>AESCTSRPHITVVEGEPFYLKHCSCSLAHEIETTTKSWYKSSGSQEHVELNPRSSSRIALHDCVLEFWPVELNDTG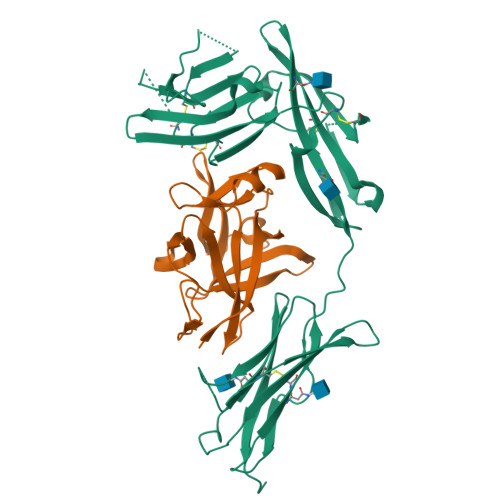SYFFQMKNYTQKWKLNVIRRNKHSCFTERQVTSKIVEVKKFFQITCENSYYQTLVNSTSLYKNCKKLLLENNKNPTIKKNAEFEDQGYYSCVHFLHHNGKLFNITKTFNITIVEDRSNIVPVLLGPKLNHVAVELGKNVRLNCSALLNEEDVIYWMFGEENGSDPNIHEEKEMRIMTPEGKWHASKVLRIENIGESNLNVLYNCTVASTGGTDTKSFILVRKADMADIPGHVFTRHHHHHH[2x];>[2x]YFGKLESKLSVIRNLNDQVLFIDQGNRPLFEDMTDSDSRDNAPRTIFIISMYKDSQPRGMAVTISVKSEKISTLSSENKIISFKEMNPPDNIKDTKSDIIFFQRSVPGHDNKMQFESSSYEGYFLASEKERDLFKLILKKEDELGDRSIMFTVQNED>MNHKVHHHHHHIEGRHMNNSGSFSLPFKLAGLGRYVPEDIVLSSELEKKYDLPQGWCLEKQGIRERRWVKGETAAFMGAEAAKEAVRDAGLQLSDIDLIISASGSPQQAVPDGGPLVQRELGLGRSGTPAITVNASCLSFFVALEVASNYLNMRRYRRILVVSADIASVSLDFRKPENFTLFGDAAAAAVVTLPEPGEKSCIHASHLRTYGFGAEFSEVRGGGSRKPPNSKDTRPEDNYLHMNGAELLKIGFEYLPKFTESLWKQCPDITVRDVKYIIPHQPSRVVLDYLSLSYPEEKLIRIIERFGNCIGASMPMALYEAVKLRGLQRGDKAVLTGTGSGVSFVGMVFTY[2x]

Myxopyronins are α-pyrone antibiotics produced by the terrestrial bacterium Myxococcus fulvus Mx f50 and possess antibacterial activity against Gram-positive and Gram-negative pathogens. Using in vitro assays we show that MxnB catalyzes a unique condensation reaction forming the α-pyrone ring of myxopyronins from two activated acyl chains in form of their β-keto intermediates. MxnB belongs to the thiolase superfamily of proteins that catalyzes the formation of carbon–carbon bonds via Claisen condensation. BLAST search results identified MxnB as a homolog of FabH, a β-ketoacyl-[acyl carrier protein (ACP)] synthase III (KAS III), highlighted by the presence of the archetypical cysteine–histidine–asparagine (CHN) catalytic triad.

MxnB crystals belonged to space group P1 and diffracted to 1.67 Å. The crystals contained one biological dimer in the asymmetric unit and the refined model includes residues 8–335 in chain A and 7–335 in chain B. The MxnB monomer displays the overall typical ketosynthase fold consisting of a five-layered core structure, α-β-α-β-α, similar to that of thiolase I.24 Although the sequence identity of MxnB to E. coli FabH is low (29%), pairwise alignment of the structures gives a Cα rmsd of just 1.5 Å over 254 (monomer) and 2.1 Å over 508 (dimer) residues, respectively. The active site of MxnB contains the catalytic CHN triad (C121, H264 and N292). The active site C121 is oxidized to cysteine sulfinic acid, but this modification appears to be either transient or a result of crystallization/data collection, since LC-MS analysis of the intact protein showed the expected mass for MxnB with unmodified cysteines. In MxnB the catalytic C121 is located at a crossroads between two substrate-binding tunnels. The first, canonical, tunnel (red) and the second (blue) tunnel, positioned as proposed for OleA, have amphipathic character (based on electrostatic surface potential maps generated in ccp4mg28). The position of the catalytic C121 in relation to both tunnel entrances strongly suggests that binding of substrate in the blue tunnel and its subsequent transacylation from the CP to MxnB C121 results in the obstruction of the red tunnel entrance. Therefore, we propose that binding of substrate in the red tunnel would have to precede binding in the blue tunnel. In agreement with the biochemical data, we propose that the western chain is preferentially delivered to and/or bound in the red tunnel, while the eastern chain is preferentially supplied via the blue tunnel.> SPNIEACGYSDRVLQLTLGNSTITTQEAANSVVAYGRWPEYLRDSEANPVDQPTEPDVAACRFYTLDTVSWTKESRGWWWKLPDALRDMGLFGQNMYYHYLGRSGYTVHVQCNASKFHQGALGVFAVPEMCLAGDSNTTTMHTSYQNANPGEKGGTFTGTFTPDNNQTSPARRFCPVDYLLGNGTLLGNAFVFPHQIINLRTNNCATLVLPYVNSLSIDSMVKHNNWGIAILPLA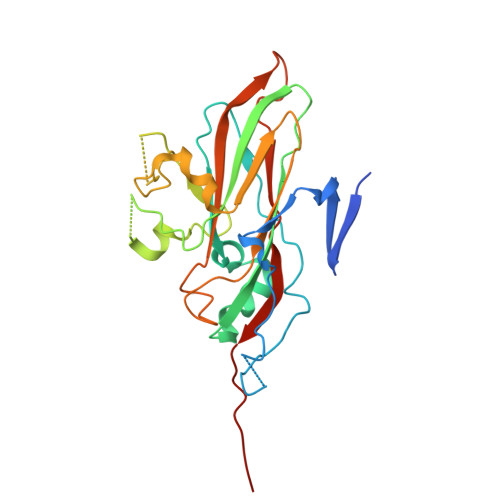PLNFASESSPEIPITLTIAPMCCEFNGLRNITLPRLQ> ALTEVEQKAANGVFDDANVQNRTLSDWDGVWQSVYPLLQSGKLDPVFQKKADADKTKTFAEIKDYYHKGYATDIEMIGIEDGIVEFHRNNETTSCKYDYDGYKILTYKSGKKGVRYLFECKDPESKAPKYIQFSDHIIAPRKSSHFHIFMGNDSQQSLLNEMENWPTYYPK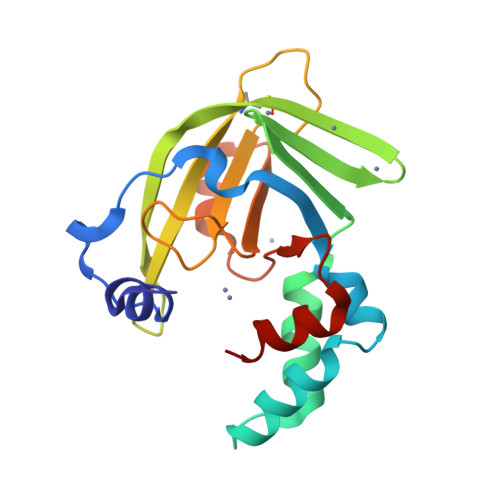QLSSEEVVEEMMS> TVPVKLKPGMDGPKVKQWPLTEEKIKALVEICTEMEKEGKISKIGPENPYNTPVFAIKKKDS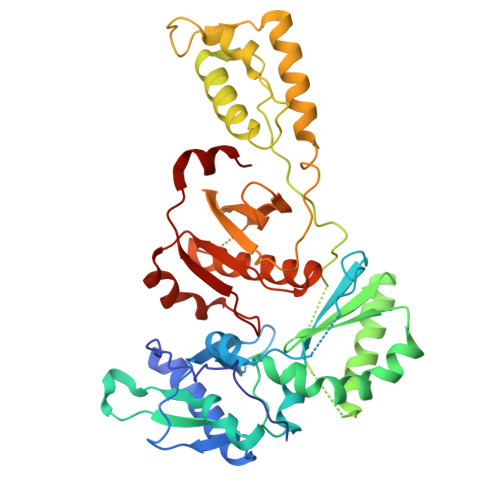TKWRKLVDFRELNKRTQDFWEVQLGIPHPAGLEKKKSVTVLDVGDAYFSVPLDEDFRKYTAFTIPSINNETPGIRYQYNVLPQGWKGSPAIFQSSMTKILEPFRKQNPDIVIYQYMDDLYVGSDLEIGQHRTKIEELRQHLLRWGLTTPDKKHQKEPPFLWMGYELHPDKWTVQPIVLPEKDSWTVNDIQKLVGKLNWASQIYPGIKVRQLCKLLRGTKALTEVIPLTEEAELELAENREILKEPVHGVYYDPSKDLIAEIQKQGQGQWTYQIYQEPFKNLKTGKYARMRGAHTNDVKQLTEAVQKITTESIVIWGKTPKFKLPIQKETWETWWTEYWQATWIPEWEFVNTPPLVKLWYQ>[4x]MSFPGWGPYPPVERDETSAITYSSKLHGSVTVRDPYSQLEVPFEDSEETKAFVHSQRKFARTYLDENPDREAWLETLKKSWNYRRFSALKPESDGHYYFEYNDGLQSQLSLYRVRMGEEDTVLTESGPGGELFFNPNLLSLDGNAALTGFV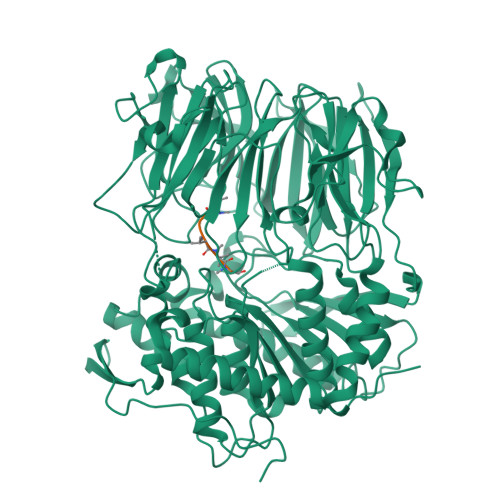MSPCGNYWAYGVSEHGSDWMSIYVRKTSSPHLPSQERGKDPGRMNDKIRHVRFFIVSWTSDSKGFFYSRYPPEDDEGKGNAPAMNCMVYYHRIGEDQESDVLVHEDPEHPFWISSVQLTPSGRYILFAASRDASHTQLVKIADLHENDIGTNMKWKNLHDPWEARFTIVGDEGSKIYFMTNLKAKNYKVATFDANHPDEGLTTLIAEDPNAFLVSASIHAQDKLLLVYLRNASHEIHIRDLTTGKPLGRIFEDLLGQFMVSGRRQDNDIFVLFSSFLSPGTVYRYTFGEEKGYRSLFRAISIPGLNLDDFMTESVFYPSKDGTSVHMFITRPKDVLLDGTSPVLQYGYGGFSLAMLPTFSLSTLLFCKIYRAIYAIPNIRGGSEYGESWHREGMLDKKQNVFDDFNAATEWLIANKYASKDRIAIRGGANGGVLTTACANQAPGLYRCVITIEGIIDMLRFPKFTFGASWRSEYGDPEDPEDFDFIFKYSPYHNIPPPGDTVMPAMLFFTAAYDDRVSPLHTFKHVAALQHNFPKGPNPCLMRIDLNSGHFAGKSTQEMLEETADEYSFIGKSMGLTMQTQGSVDSSRWSCVTV;>GFPWVIVVGVIGVIG[4x]>[32x]MKRVMIGAVAALTMLSGQALAGDAAAGQAKAAVCAACHGADG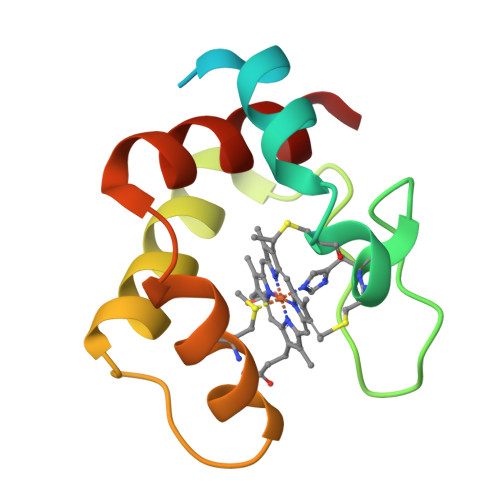NATIPGYPNLKGQNEQYIVSSIKAYKNKERSGGLAAVMQAQASLLSDDDIANLAAYYSSLK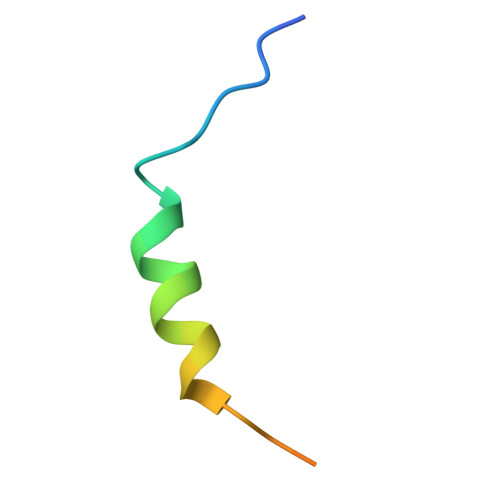> MLQFEIDDEMEPLYNQAKQMRYGDYLEVLFQ>GSHMASMKKKGSVVIVGRINLSGDTAYAQQTRGEEGCQETSQTGRDKNQVEGEVQIVSTATQTFLATSINGVLWTVYHGAGTRTIASPKGPVTQMYTNVDKDLVGWQAPQGSRSLTPCTCGSSDLYLVTRHADVIPVRRRGDSRG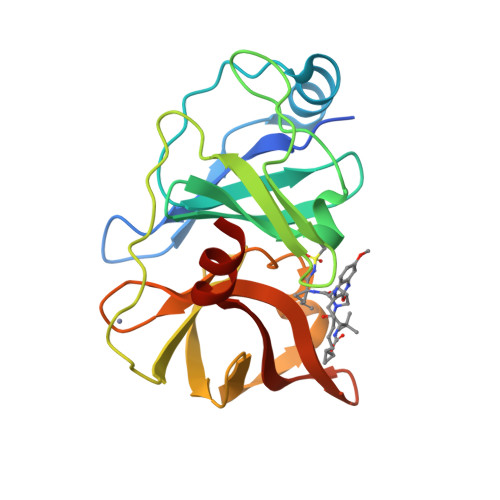SLLSPRPISYLKGSSGGPLLCPAGHAVGIFKAAVSTRGVAKAVDFIPVESLETTMRSP[4x]> GMPEDLDALLDLAARHGLDLDGGTLRTEEIGLDFRVAFARAHDGGDWVLRLPRRPDVLERAAVEGRLLAMLAPHLDVAVPDWRISTSELIAYPLLPGSPGLTVAADGEVSWHVDMASTVYARSLGSVVAQLHAVDAEAAAATGIEVRSPAQVRGAWRQDLARVGAEFEIAPALRERWEAWLADDGCWPGHSVLTHGELYPAHTLVEDERITAVLDWTTAAVGDPAKDLMFHQVSAPSAIFEVALQAYAEGGGRPWPGLARHCTEMF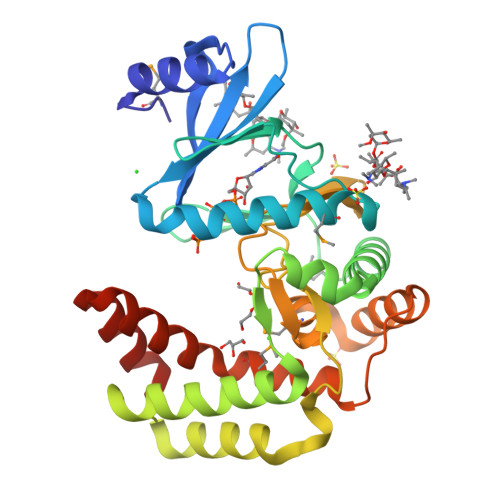SAAPLGYGLYALATGEAAHREAAAAALNPPEER> TDLPRPSISAEPGTVIPLGSHVTFVCRGPVGVQTFRLERERNYLYSDTEDVSQTSPSESEARFR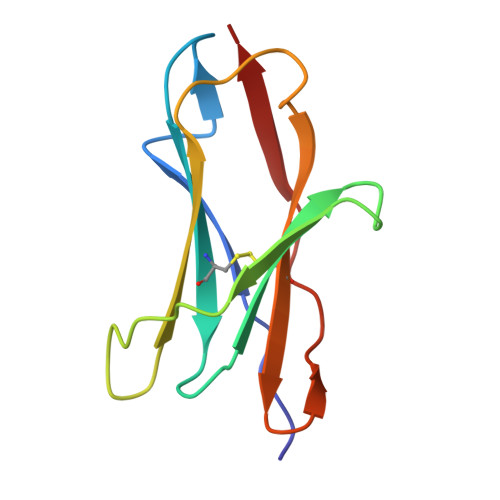IDSVNAGNAGLFRCIYYKSRKWSEQSDYLELVVK>[2x]GSMRTRVRARVISHALKDILAEGDKVIIMGHKRPDLDAIGAAIGVSRFAMMNNLEAYIVLNETDIDPTLRRVMNEIDKKPELRERFITSDDAWDMMTSKTTVVI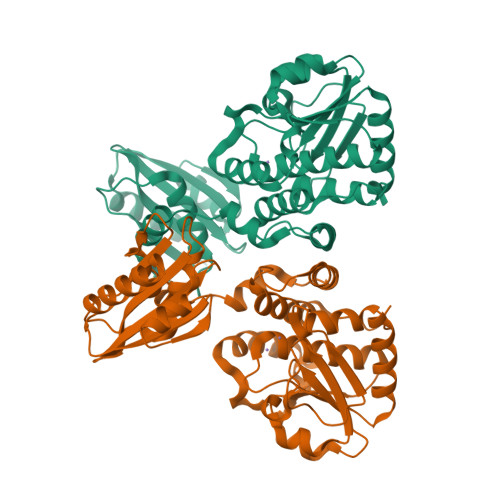VDTHKPELVLDENVLNKANRKVVIDHHRRGESFISNPLLIYMEPYASSTAELVTELLEYQPTEQRLTRLESTVMYAGIIVDTRNFTLRTGSRTFDAASYLRAHGADTILTQHFLKDDVDTYINRSELIRTVKVEDNGIAIAHGSDDKIYHPVTVAQAADELLSLEGIEASYVVARREDNLIGISARSLGSVNVQLTMEALGGGGHLTNAATQLKGVTVEEAIAQLQQAITEQLSRSEDA(3S,4S,5S,8S)-8-[(2S)-butan-2-yl]-3-methyl-3,4-bis(oxidanyl)-1-oxa-7,10-diazaspiro[4.5]decane-6,9-dione | C12 H20 N2 O5 | 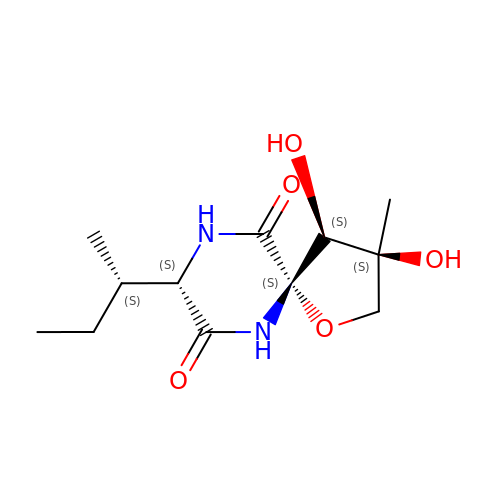AXTVENSNWFMLLA-USYUNJQESA-N>MTKRVAVIGAGPSGLAQLRAFQSAADQGAEIPEIVCFEKQANWGGLWNYTWRTGLDENGEPVHCSMYRYLWSNGPKEGLEFADYSFEEHFGKQIASYPPRAVLFDYIEGRVHKADVRKWIRFNSPVRWVSYDAETAKFTVTAHNHETDSTYSAAFDHVICASGHFSTPNVPFYEGFDTFNGRIVHAHDFRDAREFEGKDVLVMGASSSAEDIGSQCWKYGAKSITSCYRSAPMGYAWPDNWEEKPALEKLTGKTAHFADGSTRDVDAIILCTGYKHFFSFLPDDLRLKTANRL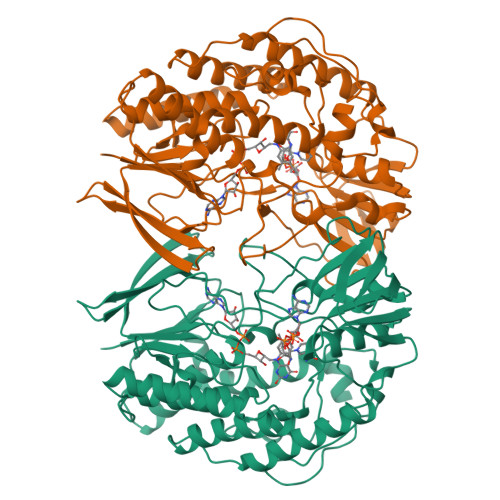ATADLYKGVAYVHNPAMFYLGMQDQWFTFNMFDAQAWWVRDAILGRITLPKDKAAMLADVAERETREEASDDVKYAIRYQADYVKELVAETDYPSFDIDGACDAFFEWKKHKAKDIMAFRDNSYKSVITGTMAPVHHTPWKEALDDSMEAYLQNHHHHHH[2x]> MKDNNPADNLAWRVIWRQLISSVGSQARMLRRSMLALLLAAFMQGIAFACLYPIIDALLRGDAPQLLNWAMAFSVAAIVTLVLRWYGLGFEYRGHLAQATHELRLRLGEQLRRVPLEKLQRGRAGEMNALLLGSVDENLNYVIAIANILLLTIVTPLTASLATLWIDWRLGLVMLLIFPLLVPFYYWRRPAMRRQMQTLGEAHQRLSGDIVEFAQGMMVLRTCGSDADKSRALLAHFNALENLQTRTHRQGAGATMLIASVVELGLQVVVLSGIVWVV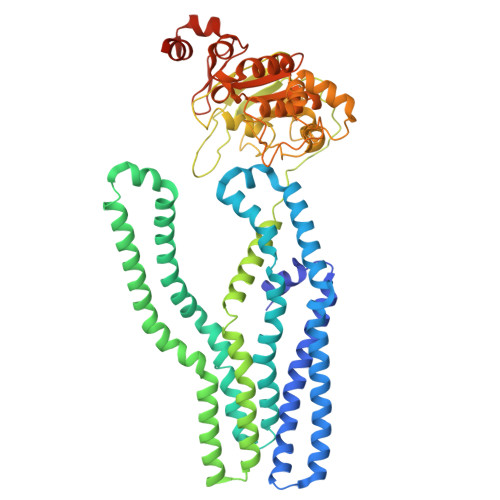TGTLNLAFLIAAVAMIMRFAEPMAMFISYTSVVELIASALQRIEQFMAIAPLPVAEQSEMPERYDIRFDNVSYRYEEGDGHALNHVSLTFPAASMSALVGASGAGKTTVTKLLMRYADPQQGQISIGGVDIRRLTPEQLNSLISVVFQDVWLFDDTLLANIRIARPQATRQEVEEAARAAQCLEFISRLPQGWLTPMGEMGGQLSGGERQRISIARALLKNAPVVILDEPTAALDIESELAVQKAIDNLVHNRTVIIIAHRLSTIAGAGNILVMEEGQVVEQGTHAQLLSHHGRYQALWQAQMAARVWRDDGGSASGEWVHE>[2x]MEFKQPNRPSYCTWELNATNSPHTCRTKNGDYTKIMPDILTAIGQTPLIKLNNIPKSYGIKCEIYAKCEFLNPGGSVKDRIAYRMIQDAEDKGLLKPGCTIIEPTSGNTGIGLAMAAAVRGYKCIIVMPEKMSDEKISTLYALGAKIIRT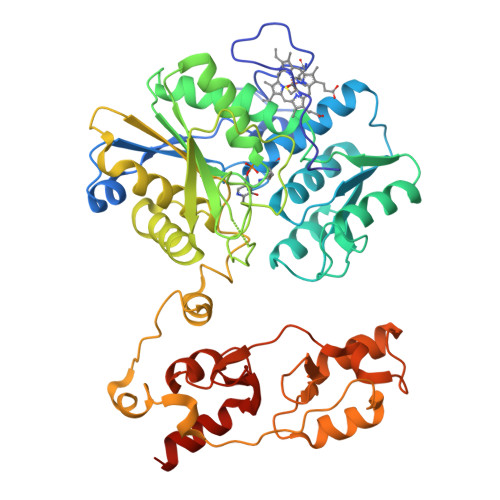PTEASWHSPEAHISVAQKLQKEIPNSIILDQYTNPGNPLAHYDQTAIEIWKQCEGKIDYLVAGAGTGGTISGIGRKLKELSPNIKIIAVDPKGSILDPSSDSQNEVGFYEVEGIGYDFIPTVLDRNVIDKWIKTEDNESLNAARMLIRQEGLLCGGSSGAALIAALKIAKDIPEEKRMVIILPDGIRNYLTKFVSEYWMETRGFLQPVCQNEMNKWWWNMKISNLSFDKQSLLKENTVTCQEAMHMLKNADSQLLVISDDNIHIKGVISLNKLTSYVISGIVKCTDFVDKAMVKQYVKVKHSATLGYISRVLEKEPYVIILDDEHDDAFIGIVNQFHILQFITKNGTSNNYLIN>MSLYKLYSMQRSGNSYKVRLALALLDAPYRAVEVDILRGESRTPDFLAKNPSGQVPLLETAPGRYLAESNAILWYLAVGTSLAPDTRMDRAEALQWMFFEQHALEPNIGSAYFWLCLVKGGRDLQTHALEDWLERGYAALQVMENHLKTNDYFAAGQLTIADIALYG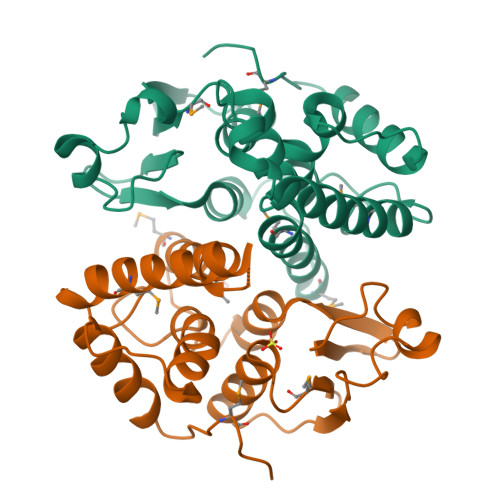YTHVADQCDFDLSTFPAVNAWLRRVEQTPGFITMDWTPETIAADPTSFAAEGHHHHHH[4x]> DPVLSEIKMPTKHHLVIGNSGDPKYIDLPEIEENKMYIAKEGYCYINIFLAMLVNVKESQAKEFTKVVRDKLVGELGKWPTLLDVATACYFLKVFYPD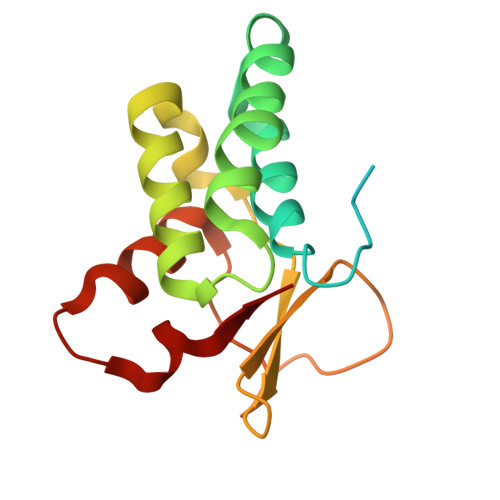VANAELPRMLVDHKTKIIHVVDSYGSLSTGYHVLKTNTVEQLIKFTRCNLESSLKHYRVG RsmI and RsmH were recently identified S-Adenosylmethionine (AdoMet)-dependent MTases responsible for the 2′-O-methylation and N4-methylation of C1402 (m4Cm1402) in bacterial 16S rRNA, respectively. The position C1402 can make direct contacts with the phosphate backbone of the P-site codon, and the modification by RsmI and RsmH plays an important role in P-site function, especially in start codon selection. RsmI is the only 2′-O-MTase among known MTases modifying bacterial 16S rRNA, and its catalytic mechanism remains unclear. The structure of RsmI monomer is composed of two independent domains: the N-terminal domain (NTD) and the C-terminal domain (CTD).

Our previous study showed the full-length RsmI was not amenable to crystallization, and the truncation Gly12-Pro258 was expressed, purified and co-crystallized with the AdoMet substrate in this study. The complex structure was solved by molecular replacement in space group C2 at a 2.20 Å resolution, and the details of data collection and structure refinement are given in Table 1. The asymmetric unit contains three RsmI molecules; two of them form a dimer formed by a noncrystallographic two-fold axis, while the third one also participates in a dimer, formed by the crystallographic two-fold axis. The crystal structure of RsmI further reveals a compact homodimer by making extensive contacts between two subunits. The two subunits interact with each other by a “back to back” mode and are nearly perpendicular with each other, and in this case the AdoMet is exposed to solvent for catalysis. AdoMet is bound into the cleft between NTD and CTD in the present complex, and the electron density for the whole AdoMet molecule was clear, therefore with well-defined conformation and orientation. AdoMet is bound tightly in a canonical conformation in the pocket which mainly consists of three loops: β1-α1 and β4-α4 from NTD domain, and β8-β9 from CTD domain, as well as sheet β7, forming a deep groove with dominantly negative charges. The direct contacts (within 3.8 Å) with AdoMet are mediated by Ile21, Thr95, Ile98 and Asp100 from NTD, and Ala124, Tyr169, Glu170, Leu198 and Met228 from CTD, with twelve H-bonds that stabilize the position and orientation of AdoMet. According to our crystal structure, we predicted the mutant D100K would abolish its side chain-mediating H-bond with AdoMet and significantly alter the surface change of AdoMet-binding pocket (from negative to positive). It was confirmed by the ITC result of D100K mutation with a complete loss of binding affinity.

>MGQLYIVPTPIGNLADITQRALEVLQAVDLIAAEDTRHTGLLLQHFGINARLFALHDHNEQQKAETLLAKLQEGQNIALVSDAGTPLINDPGYHLVRTCREAGIRVVPLPGPCAAITALSAAGLPSDRFCYEGFLPAKSKGRRDALKAIEAEPRTLIFYESTHRLLDSLEDIVAVLGESRYVVLARELTKTWETIHGAPVGELLAWVKEDENRRKGEMVLIVEGHKAQEEDLPADALRTLALLQAELP[3x]>[2x]MASQLDSGTPAREASSALRDGYRQAGVSGRVRSYLDLLAGLSDFREHFDGSDGFSLDLVDMADGPGEVTVICCAGTAAISGPHEFTRLAGALRGIAPVRAVPQPGYE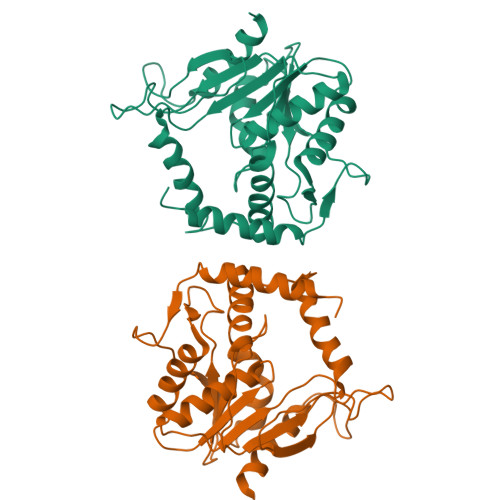EGEPLPSSMAAVAAVQADAVIRTQGDKPFVVAGHSAGALMAYALATELLDRGHPPRGVVLIDVYPPGHQDAMNAWLEELTATLFDRETVRMDDTRLTALGAYDRLTGQWRPRETGLPTLLVSAGEPMGPWPDDSWKPTWPFEHDTVAVPGDHFTMVQEHADAIARHIDAWLGGGNSSSVDKLAAALE>[2x]MLSFLLTLKRMLRAC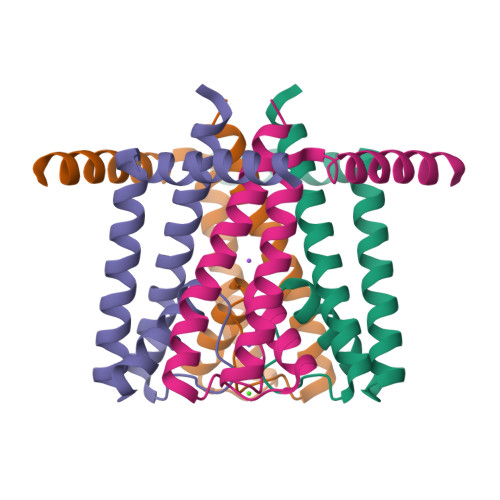LRAWKDKEFQVLFVLTILTLISGTIFYSTVEGLRPIDALYFSVVTLTTVGDGNFSPQTDFGKIFTILYIFIGIGLVFGFIHKLAVNVQLPSILSN>[4x]GAMSQIKLTPEELRSSAQKYTAGSQQVTEVLNLLTQEQAV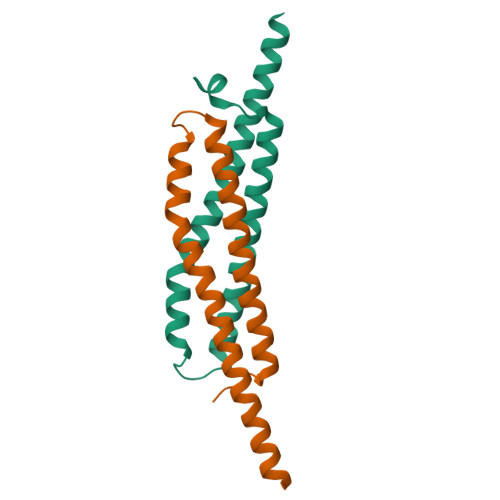IDENWDGSTFDSFEAQFNELSPKITEFAQLLEDINQQLLKVADIIEQTDADIASQISG>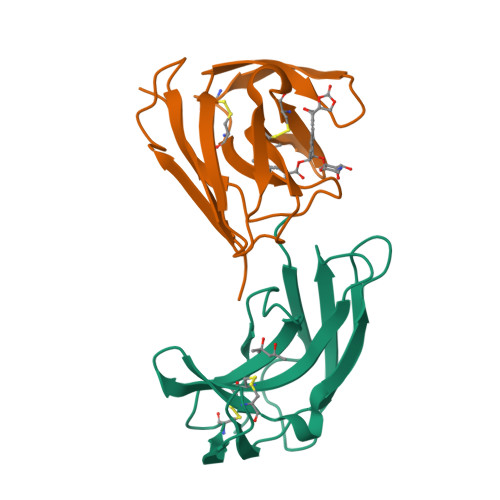[2x]AAPTATVTPSSGLSDGTVVKVAGAGLQAGTAYDVGQCAWVDTGVLACNPADFSSVTADANGSASTSLTVRRSFEGFLFDGTRWGTVDCTTAACQVGLSDAAGNGPEGVAISFN>[2x]SPITGLVYDQRMMLHHNMWDSHHPELPQRISRIFSRHEELRLLSRCHRIPARLATEEELALCHSSKHISIIKSSEHMKPRDLNRLGDEYNSIFISNESYTC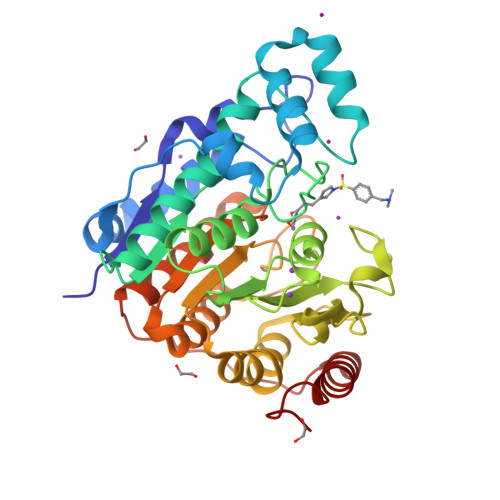ALLAAGSCFNSAQAILTGQVRNAVAIVRPPGHHAEKDTACGFCFFNTAALTARYAQSITRESLRVLIVDWDVHHGNGTQHIFEEDDSVLYISLHRYEDGAFFPNSEDANYDKVGLGKGRGYNVNIPWNGGKMGDPEYMAAFHHLVMPIAREFAPELVLVSAGFDAARGDPLGGFQVTPEGYAHLTHQLMSLAAGRVLIILEGGYNLTSISESMSMCTSMLLGDSPPSLDHLTPLKTSATVSINNVLRAHAPFWSSLR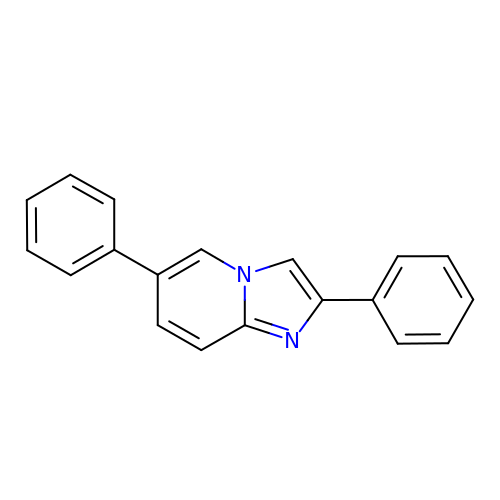2,6-diphenylimidazo[1,2-a]pyridine | C19 H14 N2 | LETMYYZWCFHZLY-UHFFFAOYSA-N> SPNVEACGYSDRVQQITLGNSTITTQEAANAVVCYAEWPEYLP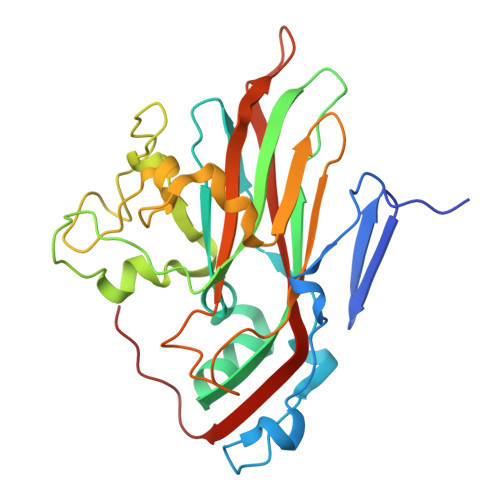DVDASDVNKTSKPDTSVCRFYTLDSKTWTTGSKGWCWKLPDALKDMGVFGQNMFFHSLGRSGYTVHVQCNATKFHSGCLLVVVIPEHQLASHEGGNVSVKYTFTHPGERGIDLSSAADTIGPGRAFYTTKNNEVGGPVKDVIYNMNGTLLGNLLIFPHQFINLRTNNTATIVIPYINSVPIDSMTRHNNVSLMVIPIAPLTVPTGATPSLPITVTIAPMCTEFSGIRSKSIVPQ> QDSRRSA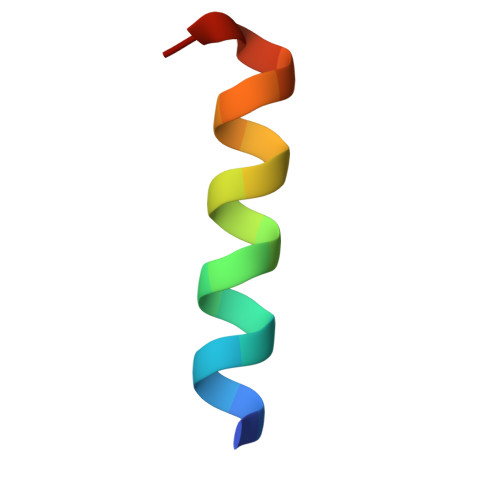DALLRLQAMAGIS>MARKYFVAANWKCNGTLESIKSLTNSFNNLDFDPSKLDVVVFPVSVHYDHTRKLLQSKFSTGIQNVSKFGNGSYTGEVSAEIAKDLNIEYVIIGHFQRRKYFHETDEDVREKLQASLKNNLKAVVCFGESLEQREQNKTIEVITKQVKAFVDLIDNFDNVILVYEPLWAIGTGKTATPEQAQLVHKEIRKIVKDTCGEKQANQIRILYGGSVNT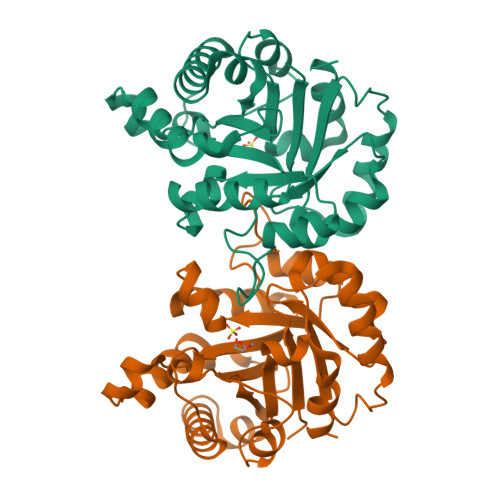ENCSSLIQQEDIDGFLVGNASLKESFVDIIKSAM[2x]>MISHSELRKLFYSADAVCFDVDSTVIREEGIDELAKICGVEDAVSEMTRRAMGGAVPFKAALTERLALIQPSREQVQRLIAEQPPHLTPGIRELVSRLQERNVQVFLISGGFRSIVEHVASKLNIPATNVFANRLKFYFNGEYAGFDETQPTAESGGKGKVIKFLKEKFHFKKIIMIGD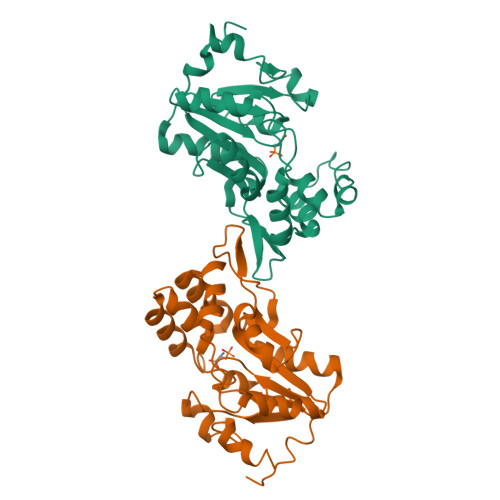GATDMEACPPADAFIGFGGNVIRQQVKDNAKWYITDFVELLGELEE[2x]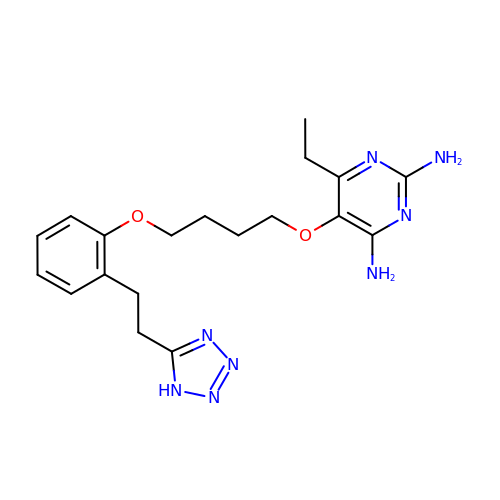6-ethyl-5-(4-{2-[2-(1H-tetrazol-5-yl)ethyl]phenoxy}butoxy)pyrimidine-2,4-diamine | C19 H26 N8 O2 | OUJSJGDTRMGLDA-UHFFFAOYSA-N>[12x]MASISEKMVEALNRQINAEIYSAYLYLSMASYFDSIGLKGFSNWMRVQWQEELCH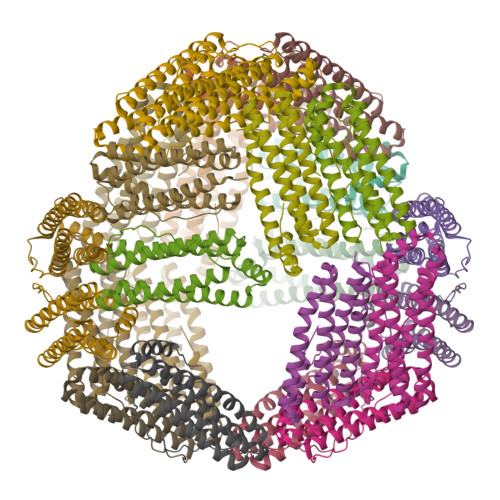AMKMFDFVSERGGRIFLQDIKKPDSEWESPLAAFEHVYEHEVNVTKRIHELVEMAMQEKDFATYNFLQWYVAEQVEEEASALDIVEKLRLIGEDKRALLFLDKELSLRQFTPPAEEEK>PDLYYVPGSAPCRAVLLTAKALNLNLNLKLVDLHHGEQMKPEYLKLNPQHTVPTLVDDGLAIAESRAILTYLVNKYGKGSTLYPEDPKARAIVDQRLYFDIGTLYQRFGDYFYPQLFGGAPEDKEKL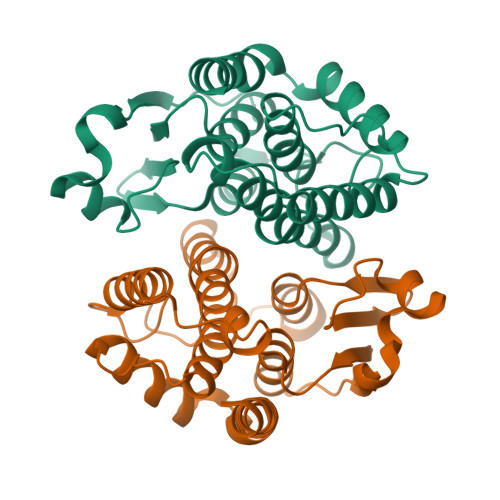AKVDEALKFLDTFLEGQKYVAGNNLTVADLSLVASVSSFEAANIDFLKYGNVKRWYETVKATAPGYEEANGKGLEAFKGLVNSIM[2x]> MARYTMTLYDFIKSELIKKGFNEFVNDNKLTFYDDEFQFMQKMLKFDKDVLAIVNEKVFK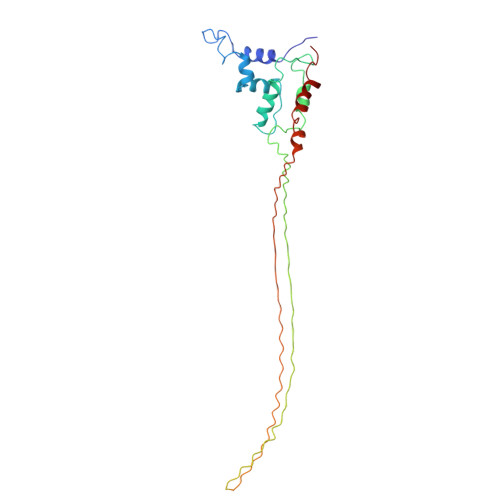GFSLKDELSDLLFKKSFTIHFLDREINRQTVEAFGMQVITVCITHEDYLNVVYSSSEVEKYLQSQGFTEHNEDTTSNTDETSNQNATSLDNSTGMTANRNAYVSLPQSEVNIDVDNTTLRFADNNTIDNGKTVNKSSNESNQNAKRNQNQKGNAKGTQFTKQYLIDNIDKAYDLRKKILNEFDKKCFLQIW> EINQPSILVLKEDENATLSCRQNDNHDYMSWYLQQPGKGLQLIYSSYGVKQENKGDIHTGYEAKRSSQEVFHLDIISAKKNHSAIYFCASS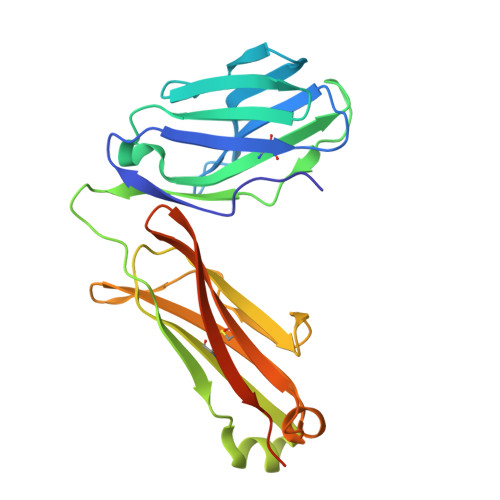SYKGNTPLNFGQGTRLTVLGKNSEIIEPDVVIFSPSKQEIQEKKKATLVCLASGFFPDHLNLVWKVNGVKRTEGVGTDEISTSNGSTYSLTSRLRISAQEWFNPLNRFECIANFFKNGTQQSIQKIIYGDTGCDIFKENYQRSATAGK Inhibitory family members typically fold to a metastable native state that undergoes a major conformational change (termed the stressed [S] to relaxed [R] transition) central for the protease inhibitory mechanism. In previous work, we designed and characterized conserpin, a synthetic serpin that folds reversibly, is functional, thermostable and resistant to polymerization. Conserpin was designed using consensus engineering, using a sequence alignment of 212 serpin sequences and determining the most frequently occurring amino acid residue at each position. The reactive center loop (RCL) protrudes from the main body of the molecule and contains the scissile bond (P1 and P1’ residues), which mediates α1-AT’s inhibitory specificity against the target protease, neutrophil elastase (HNE).

With the aim of changing the specificity of conserpin to that of α1-AT, a conserpin/α1-AT chimera was previously produced, where 9 residues within the RCL (P7-P2’) were swapped with the corresponding residues from α1-AT. The resulting chimera, conserpin-AATRCL (379 aa) has a 61% sequence identity with α1-AT (148 residue differences). To understand if there are any structural changes caused by modifying the RCL, we determined the x-ray crystal structure of conserpin-AATRCL in the native state. The overall structure of conserpin-AATRCL is identical to that of conserpin—a structural alignment reveals a root mean square deviation (RMSD) of 0.2 Å across all Cα atoms. Like conserpin and indeed many other serpins, the RCL of conserpin-AATRCL is too flexible to be modelled into the electron density. Importantly, conserpin-AATRCL does not inhibit HNE, the protease target of α1-AT. SDS-PAGE using 1:1 and 2:1 serpin: protease molar ratios reveals a faint complex between conserpin-AATRCL and HNE, but also showed a large amount of cleaved species compared to the complex formation between α1-AT and HNE. In comparison, the formation and stability of a complex may be hindered by the charge−charge repulsion between the electropositive S3–S4 binding pockets of HNE and the electropositive surface of P6−P3 of the RCL. Despite P7-P2’ of conserpin-AATRCL being identical to the corresponding region in α1-AT, the overall flexibility of the RCL region as a whole was not reduced to the level of α1-AT, while the hinge region of the RCL, which inserts into β-sheet A first during insertion, exhibited higher flexibility in conserpin-AATRCL compared to α1-AT.

> MHHHHHHENLYFQGAASSHKLAEANTDFAFSLYRELAKSSPDKNIFFSPVSISSALAMLSLGAKGDTHTQILEGLGFNSEADIHQGFQHLLQTLNRPKGLQLKTANGLFVDKSLKLLDSFLEDSKKLYQAEAFSVDFDPEEAKKQINDWVEKQTNGKIKDLLKDLDSDTVLVLVNAIYFKGKWKKPFDPENTKEEDFHVDEKTTVKVPMMSQKGKFYYYHDDELSCKVLELPYKGNASMLIILPDEGGLQHLEQSLTPETLSKWLKSLTRRSVELYLPKFKIEGTYDLKEVLSNLGITDLFSPGADLSGITEEKLYVSKAVHKAVLEVNEEGTEAAAATFLEAIPMSIPPEFKADRPFLFLIRENKTGSILFMGKVVNP(1R)-1-phenylethane-1,2-diol | C8 H10 O2 | 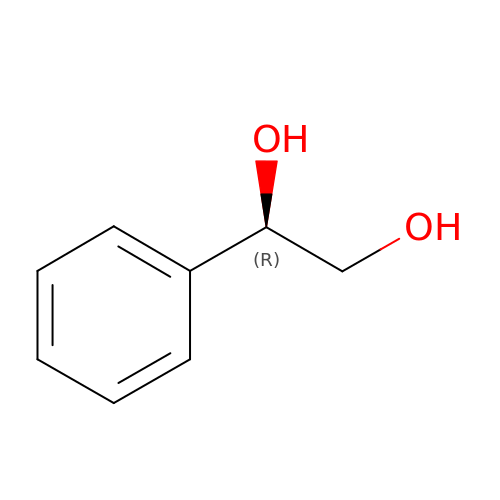PWMWNFMRSKOCEY-QMMMGPOBSA-N In Pseudomonas aeruginosa, the Xcp T2SS plays an important role in bacterial virulence by its capacity to deliver a large panel of toxins and degradative enzymes into the surrounding environment. Secretins are large homooligomeric assemblies of 12 to 16 monomers forming a distinctive bipartite ring-shaped and cylindrical structure on their C- and N-terminal sides, respectively. The periplasmic N domain of secretins is constituted by the succession of structurally independent subdomains labeled N0 to N3 (7–9). Here, we revealed that the N-terminal domain of the T2SS secretin XcpQ from Pseudomonas aeruginosa is able to self-assemble into a hexamer of dimers independently of its C-terminal domain.

To gain deeper structural information on XcpQN012 multimerization, we endeavored to determine the 3D structure of the purified recombinant XcpQN012 by X-ray crystallography. The overall structure of the XpQN012 monomer, refined at 3.0-Å resolution, showed a typical organization into three subdomains, N0, N1, and N2, where each subdomain abuts the next in an N0:N1:N2 arrangement in three dimensions. The crystal structure revealed an axial dimeric association of XcpQN012 organized in face-to-face fashion. The dimer packing is stabilized by the interaction between N0-N0* and N2-N2* subdomains from each monomer (the “*” corresponds to the second molecule in the dimer). The dimerization seems to be driven by the N2-N2* contact with a buried surface of 600 Å2 that represents about 60% of the total buried surface. Most of the contacts between N2 subdomains are localized within the β9 strand interacting with the β9* in the facing N2* subdomain, creating a continuous 6-stranded antiparallel β-sheet. In contrast to XcpQN012, the N2 subdomain of GspD is not in contact with the N1 subdomain. This difference results in a high root mean square deviation (RMSD) (4.36 Å) when the two structures are superimposed. However, a slight difference was observed between the packing of the two XcpQ dimers, due to a general displacement of monomer B toward monomer A. This leads, in the present study, to a more compact dimer with a larger buried surface area of 1,040 Å2 compared to 880 Å2 for the previous structure.

>ENSGGNAFVPAGNQQEAHWTINLKDADIREFIDQISEITGETFVVDPRVKGQVSVVSKAQLSLSEVYQLFLSVMSTHGFTVVAQGDQARIVPNAEAKTEAGGGQSAPDRLETRVIQVQQSPVSELIPLIRPLVPQYGHLAAVPSANALIISDRSANIARIEDVIRQLDQKGSHDYSVINLRYGWVMDAAEVLNNAMSRGQAKGAAGAQVIADARTNRLIILGPPQARAKLVQLAQSLDTPT[2x]Rspo (R-spondin, also roof plate-specific spondin) proteins are evolutionarily conserved from fish to humans and have well-documented roles in a broad range of developmental and physiological processes resulting from enhancement of canonical and non-canonical Wnt signalling. ZNRF3/RNF43 specifically targets these Wnt receptors for ubiquitination and turnover, hence reducing Wnt signalling responses. Direct extracellular interaction with Rspo proteins inhibits ZNRF3/RNF43 activity. Here we report a molecular level analysis of the ZNRF3/RNF43 ectodomain structure and its interactions with Rspo proteins.

By using a combination of heavy atom and molecular-replacement-based phasing strategies, we determined multiple crystal structures for Xenopus (x) Rspo2Fu1–Fu2 (highest resolution 2.2 Å), xZNRF3ecto, zebrafish (z) ZNRF3ecto and mouse (m) ZNRF3ecto, (highest resolutions 2.4, 1.6 and 2.0 Å, respectively), plus complexes comprising xZNRF3ecto–xRspo2Fu1–Fu2, mZNRF3ecto–mRspo2Fu1–Fu2, mZNRF3ecto–xRspo2Fu1–Fu2 and xRNF4F3ecto–xRspo2Fu1–Fu2 (at 2.1, 2.8, 2.4 and 2.7 Å, respectively). The crystal structures of the ZNRF3ecto–Rspo2Fu1–Fu2 and RNF43ecto–Rspo2Fu1–Fu2 complexes revealed a 1:1 interaction between Fu1 of the Rspo2Fu1–Fu2 and a single ZNRF3ecto or RNF43ecto chain. The first, extensive, area of interaction involves hydrophobic interactions interspersed with hydrophilic (complementarily charged) patches contributed by the first two β-hairpins of the Rspo Fu1 and the region immediately carboxy-terminal to the β3 strand of ZNRF3ecto. The Met-finger at the tip of the second β-hairpin of Fu1 nestles into a pocket formed between the β3 strand and the αC–β7 loop of the ZNRF3ecto, which is lined with hydrophobic residues (I95, I191, V192, A198). The αC–β7 loop is a flexible region in the unliganded ZNRF3ecto crystal structures and moulds to interface the RspoFu1–Fu2 M68 in the complex. The acidic region of the β3–β4 loop (immediately adjacent to C104 of the disulphide bridge) becomes more ordered in the ligand-bound ZNRF3ecto structures, probably as a result of electrostatic interactions with a positively charged patch on Rspo Fu1. For all ZNRF3ecto–Rspo2Fu1–Fu2 complex structures we determined (from five different combinations of species and crystal forms), the dimer found in most of the unliganded ZNRF3ecto crystal structures reoccurs. The overall assembly thus comprises a 2:2 complex of ZNRF3ecto–Rspo2Fu1–Fu2. The 2:2 complex resembles a crab with the ZNRF3ecto dimer forming the body from which the two Rspo2Fu1–Fu2 ligands diverge, without interacting with each other, as the pincers. Notably, the β1–β2 hairpin shows less conformational variation in the liganded ZNRF3ecto dimer structures, always maintaining a tight embrace, consistent with the Rspo2Fu1–Fu2 interactions contributing an indirect stabilizing effect on the dimer via the β3–β4 loop.

>[2x]ETGKETAFVEVVLFESSPSGDYTTHTTGLTGRFSRAGAMLSAEGEIVQMHPLGLCNNNDEEDLYEYGWVGVVKLEQPELDPKPCLTVLGKAKRAVQRGATAVIFDVSENPEAIDQLNQGSEDPLKRPVVYVKGADAIKLMNIVNKQKVARARIQHLGTKHHHHHH;>ETGGTNPICKGCLSCSKDNGCLRCQPKLFFYLRREGMRQYGECLQSCPPGYYGVRGPDMNRCSRCRIENCDSCFSRDFCIKCKSGFYSHKGQCFEECPEGFAPLDDTMVCVDGTKHHHHHH[2x]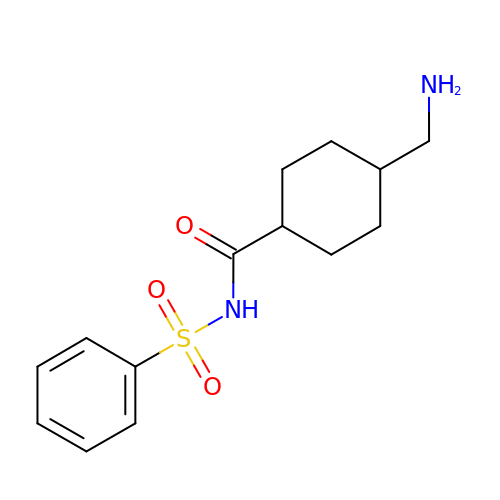4-(aminomethyl)-N-(benzenesulfonyl)cyclohexanecarboxamide | C14 H20 N2 O3 S | BCEUUNKKXUMFST-HAQNSBGRSA-N>[10x]MTEAQAIAKQLGGVKPDDEWLQAEIARLKGKSIVPLQQVKTLHDWLDGKRKARKSCRVVGESRTGKTVACDAYRYRHKPQQEAGRPPTVPVVYIRPHQKCGPKDLFKKITEYLKYRVTKGTVSDFRDRTIEVLKGCGVEMLIIDEADRLKPETFADVRDIAEDLGIAVVLVGTDRLDAVIKRDEQVLERFRAHLRFGKLSGEDFKNTVEMWEQMVLKLPVS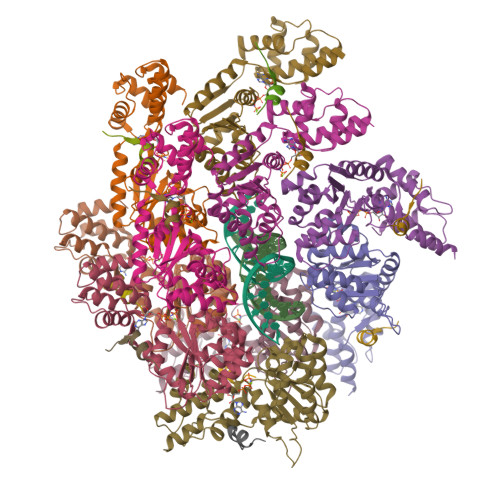SNLKSKEMLRILTSATEGYIGRLDEILREAAIRSLSRGLKKIDKAVLQEVAKEYK;>[10x]IEVWDYEQLREEYGF>MAHHHHHHMNFQRMTDLNLAGKRVLIREDLNVPVKNGVITSDARLRAALPTIKAALEKGAAVMVFSHLGRPVEGEPKPEQSLAPVAAYLTEALGQEVKLFTDYLDGVEVEAGQVVLLENVRFNPGEKKNNPELAQKYAALCDVFVMDAFGTAHRAEASTEGVARFAPVAAAGPLLAAELDALGRAMQTPEKPMVAIVAGSKVSTKLDVLNSLSGICDQLIVGGGIANTFLAAAGYNVGKSLYEADLVETAKQIAAKVSVPLPTDVVVADASQINFEDFLGSLAAAQAVIKKVEDVTANDMILDVGPETAKAFANILTTS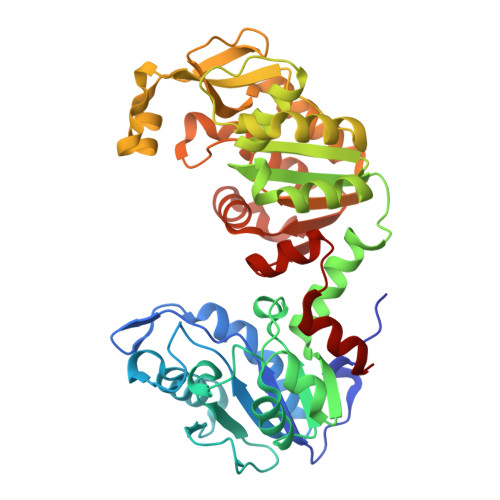KTILWNGPVGVFEVDQFGEGTKALSLAVAQSDAFSIAGGGDTLAAIDKYNVADQIGYISTGGGAFLEFVEGKTLPAVAVLLERA[6x]> MSELEKAVVALIDVFHQYSGRE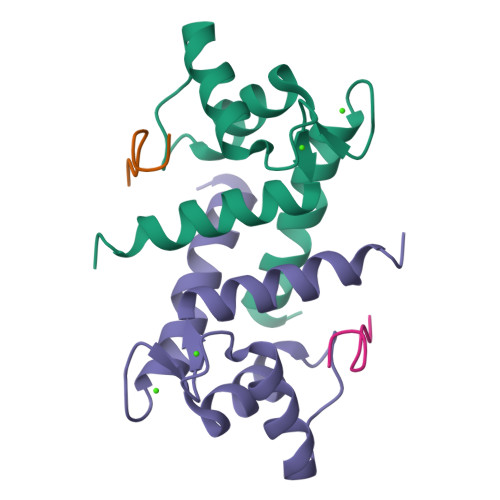GDKHKLKKSELKELINNELSHFLEEIKEQEVVDKVMETLDSDGDGECDFQEFMAFVAMITTACHEFFEHE;> TRTKIDWNKILS>MGKLVLYGIDPSPPVRACLLTLKALNLPFEYKVVNLFAKEHLSEEYLKKNPQHTVPTLEEDGHLIWDSHAIMAYLVSKYGKDDSLYPKDLLKRAVVDQRMYFEAGVLFQGGLRNITAPLFFRNQTQIPQHQIDSIVESYGFL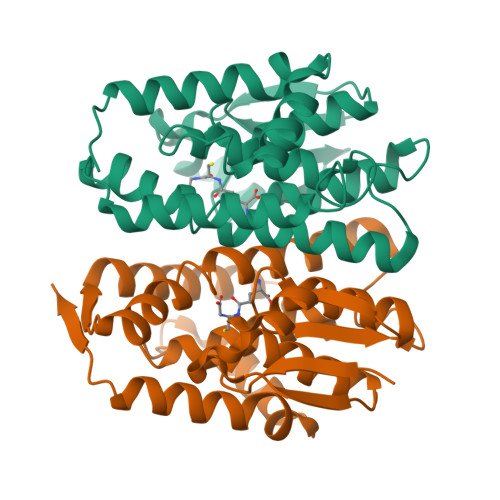ESFLKNNKYMAGDHLTIADFSIVTSVTSLVAFAEIDQSKFPKLSAWLKSLQSLPFYEEANGAGAKQLVAMVKSKNLTIVP[4x]TcSMP is a poorly characterized protein, reported to be involved in mammalian cell invasion, with an auxiliary role to gp82, the major adhesion protein of metacyclic trypomastigotes. It is highly conserved among different Trypanosoma spp., making it an ideal candidate for CD diagnosis. To date, the function of TcSMP remains to be elucidated; however, knock-out studies carried out on a homologous antigen (43.7% sequence identity) from T. brucei (procyclic-specific surface antigen-2; TbPSSA) underlined the importance of the protein for parasite transmission. In this context, we describe the production and high-resolution (1.62 Å) crystal structure determination of a surface membrane protein from T. cruzi (TcSMP) as a potential serodiagnostic antigen for structure-based in silico epitope mapping and design.

The crystal structure of TcSMP was solved at 1.62 Å resolution. Crystals belonged to the monoclinic C2 space group, with one molecule in the asymmetric unit and a Matthews coefficient of 2.01 Å3/Da (estimated solvent content of 39.5%). Overall, the electron density map was of good quality, covering residues from 41 to 254 with no gaps. The 3D crystal structure of TcSMP displayed an elongated, “C-shaped” architecture, comprising two lobes (lobes 1 and 2), linked together by a flexible hinge region. Overall, the structure was found to be composed of 12 β-strands and 5 short α-helices with an elongated strand (β9) that stretches from lobe 2 across to lobe 1. The larger lobe, lobe 1, comprised residues from both the amino and carboxy termini, and hosted most of the secondary structural elements of the protein. Lobe 2 comprised β-strands β7, β8, and β11 and the elongated connector β9 strand, plus helices α3 and α4. Strands β7, β8, and β9 formed an antiparallel β-sheet. This lobe was found to be stabilized by intra-molecular hydrogen bonds between residues coming from β7 and β9 strands, as well as by three disulfide bridges, formed by C139–C145, C158–C181, and C172–C178. As determined by the secondary structure matching (SSM) program in Coot, superposition with the T. brucei antigen revealed a high degree of structural similarity (RMSD of 1.9 Å over 162 aligned Cα atoms), with large differences only in the lobe 2 region, whereas structural alignment with the antigen from T. congolense resulted in an overall higher RMSD value (3.3 Å) with major deviations in lobe 2 and helices α1 and α5 of lobe 1. Two separate, sequential linear epitopes (Ep1: residues 130 to 156; Ep2: residues 163 to 182) were predicted and located to lobe 2.

> MCLFGIVDAVADFLKGVVACACCLIIGGPALIIAGSMLLNQQDLRKAFRDAVNEFNPTPMNAWTGTINDVPIAVRRESLNVKGVDGATSVFAEAVVSVSHMSSSRFQVSVNVRTVTPFNRMAPFRTIEKTSYTCSSRDCKSRLNCQCNELLNSFMNQCVASGGKFVRTPGMCVLDRTCGTCERTVYLRQLYLVVREVSNGKYAEDTNLRSAMYAFGDLDNDYQPGIPSTVTVRLYSSKDPYIALQRLTKGTNDLGLNSRTVGIVLIVLGCLFLLLEIGVCTALICYWMRRKKTSSGAPPYMAPATYGISNSGASGNAAPNFYAQPAQQTGQGYTYFQAAPPGYTYGQPPQGQPVPQGYAYGQPVSPQGQHGYTYGQAPPPLYAYGQPVSPQAPRGQVPPPL> MKSSHHHHHHENLYFQSNAESYTLTPEVGELIEKVRKAHQETFPALCQLGKYTTNNSSEQRVSLDIDLWDKFSELSTKCIIKTVEFAKQLPGFTTLTIADQITLLKAACLDILILRICTRYTPEQDTMTFSDGLTLNRTQMHHAGFGPLTDLVFAFANQLLPLEMDDAETGLLSAICLICGDRQDLEQPDRVDMLQEPLLEALKVYVRKRRP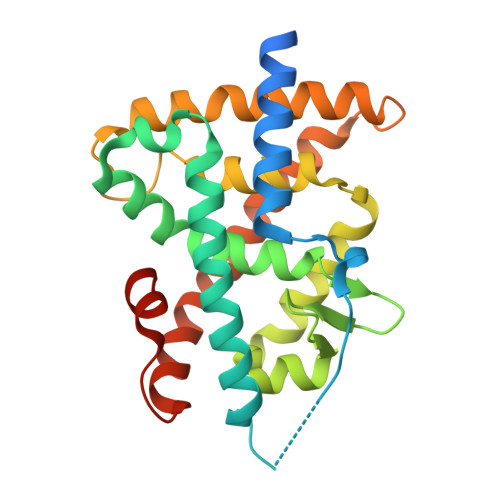SRPHMFPKMLMKITDLRSISAKGAERVITLKMEIPGSMPPLIQEMLENSEGLD>[2x]GSTGSMVKSGKARAHTNIALIKYWGKADETYIIPMNNSLSVTLDRFYTETKVTFDPDFTEDCLILNGNEVNAKEKEKIQNYMNIVRDLAGNRLHARIESENYVPTAAGLASSASAYAALAAACNEALSLNLSDTDLSRLARRGSGSASRSIFGGFAEWEKGHDDLTSYAHGINSNGWEKDLSMIFVVINNQSKKVSSRSGMSL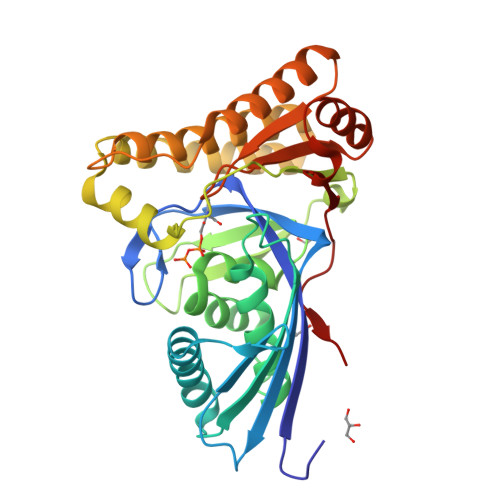TRDTSRFYQYWLDHVDEDLNEAKEAVKNQDFQRLGEVIEANGLRMHATNLGAQPPFTYLVQESYDAMAIVEQCRKANLPCYFTMAAGPNVKVLVEKKNKQAVMEQFLKVFDESKIIASDIISSGVEIIK> SIFSYI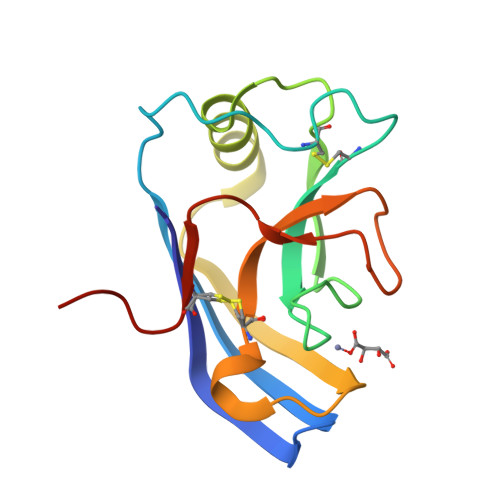TESTGTPSNATYTYVIERWDPETSGILNPCYGWPVCYVTVNHKHTVNGTGGNPAFQIARIEKLRTLAEVRDVVLKNRSFPIEGQTTHRGPSLNSNQECVGLFYQPNSSGISPRGKLLPGSLCGAHHHHHH Multifunctional collagen lysyl hydroxylases (LHs/PLODs) possess both Fe2+-dependent lysyl hydroxylase (LH) and Mn2+-dependent glucosyltransferase activities. LH3/PLOD3 is thought to be capable of performing two chemically distinct collagen glycosyltransferase reactions using the same catalytic site: an inverting beta-1,O-galactosylation of hydroxylysines (Gal-T) and a retaining alpha-1,2-glucosylation of galactosyl hydroxylysines (Glc-T). In this work, we have combined indirect luminescence-based assays with direct mass spectrometry-based assays and molecular structure studies to demonstrate that LH3/PLOD3 only has Glc-T activity and that GLT25D1 only has Gal-T activity. The LH3/PLOD3 N-terminal GT domain shares its fold with Mn2+-dependent GT-A glycosyltransferases, encompassing a UDP-donor substrate binding cavity stretched towards a catalytic pocket.

Aiming to further elucidate the significance of the differences caused by this specific residue in LH1/PLOD1 and LH3/PLOD3, we generated a LH3/PLOD3 p.(Asp190Ser) variant to mimic LH1/PLOD1 at that specific site. MS and luminescence data showed that this single-point mutation completely abolishes the LH3/PLOD3 Glc-T activity without affecting the ability of this mutant to bind UDP-Glc donor substrates. We also solved the 2.30-Å crystal structure of the full-length human LH3/PLOD3 p.(Asp190Ser) mutant in complex with Mn2+ and UDP-Glc. Overall, the structure appeared nearly identical to wild-type LH3/PLOD3. Analysis of the electron density at the GT catalytic site showed clear signals for the Glc moiety of the UDP-Glc donor substrate. This feature was never observed when using wild-type LH3/PLOD3, further supporting the importance of the Poly-Asp loop for Glc-T activity. The side chains of Asp191, Lys89, and Ser166, as well as the main chain carbonyl of Thr83, were found at distances and orientations possibly compatible with electrostatic contacts with the Glc moiety of the donor substrate, resulting in the trapping of the sugar in a portion of the catalytic cavity, leaving a large pocket shaped by residues Glu141, Phe143, Asn165, Asn223, and Asn255 available to likely host the Gal moiety of the acceptor substrate for catalysis. LH3/PLOD3 p.(Asp190Ser), matching the corresponding residue in LH1/PLOD1, resulted in strongly diminished Glc-T activity and yielded a crystal structure with observable electron density for the donor sugar moiety for the first time, enabling the identification of the amino acid residues directly involved in Glc binding and those shaping the portion of the cavity likely hosting the Gal moiety of the acceptor substrate. Whilst co-crystal structures with donor substrate consistently display no density for the sugar moiety because of uncoupled enzymatic hydrolysis or very low occupancy for a very flexible moiety, the inhibitors show density for the glycan part connected to UDP because hydrolysis is not taking place.

> GSSDRPRGRDPVNPEKLLVITVATAETEGYLRFLRSAEFFNYTVRTLGLGEEWRGGDVARTVGGGQKVRWLKKEMEKYADREDMIIMFVDSYDVILAGSPTELLKKFVQSGSRLLFSAESFCWPEWGLAEQYPEVGTGKRFLNSGGFIGFATTIHQIVRQWKYKDDDSDQLFYTRLYLDPGLREKLSLNLDHKSRIFQNLNGALDEVVLKFDRNRVRIRNVAYDTLPIVVHGNGPTKLQLNYLGNYVPNGWTPEGGCGFCNQDRRTLPGGQPPPRVFLAVFVEQPTPFLPRFLQRLLLLDYPPDRVTLFLHNNEVFHEPHIADSWPQLQDHFSAVKLVGPEEALSPGEARDMAMDLCRQDPECEFYFSLDADAVLTNLQTLRILIEENRKVIAPMLSRHGKLWSNFWGALSPDEYYARSEDYVELVQRKRVGVWNVPYISQAYVIRGDTLRMELPQRDVFSGSDTDPDMAFCKSFRDKGIFLHLSNQHEFGRLLATSRYDTEHLHPDLWQIFDNPVDWKEQYIHENYSRALEGEGIVEQPCPDVYWFPLLSEQMCDELVAEMEHYGQWSGGRHEDSRLAGGYENVPTVDIHMKQVGYEDQWLQLLRTYVGPMTESLFPGYHTKARAVMNFVVRYRPDEQPSLRPHHDSSTFTLNVALNHKGLDYEGGGCRFLRYDCVISSPRKGWALLHPGRLTHYHEGLPTTWGTRYIMVSFVDPAAA Human Caprin family comprises two members, Caprin-1 and Caprin-2. Previously, we reported Caprin-2 as a new regulator of canonical Wnt signaling through a mechanism of facilitating LRP5/6 phosphorylation. HR1 domain is so far only observed in Caprin-1 and Caprin-2, and this domain shares no sequence similarities with any other known motifs, indicating that HR1 may perform a unique function.

We then tried the corresponding region of hCap2_HR1 (aa S102–K351) based on sequence alignment between hCaprin-2 and zCaprin-2, and this hCap2_HR1 protein was crystallized with significantly improved diffractions. Two molecules of hCap2_HR1 form an asymmetric dimer, with the overall structure roughly resembling the shape of a pair of "scissors" measuring ∼100 Å in height and ∼60 Å in width. The structure of hCap2_HR1 could be divided into two subdomains: a "blade"-like N-lobe (aa A112-L205) and a "bow"-like C-lobe (aa K206-P320). The parts of helices α3-2 and α3′ in the C-lobe of chains A and B, respectively, packed together forming a parallel coiled-coil dimer with the rest helices in the N-lobe forming two antiparallel dimers. The dimeric interface has a total buried area of 2414.4 Å2. Considering the theoretical MW of Cap2_HR1 being 29.2 kDa, we tend to conclude that Cap2_HR exists as a dimer in solution. Close to the junction of the N-lobe and the C-lobe, a cluster of basic residues aligned along the solve-exposed side of the coiled coil of the N-lobe. Surprisingly, we found that Cap2_HR1 binds specifically to phosphatidylinositol 4-phosphate (PI4P), and mutations targeting R200 and R201 in this basic cluster not only disrupt Caprin-2's association with PI4P but also lead to altered cellular localization as well as decreased activities of Caprin-2 in canonical Wnt signaling. WT hCap2_HR1 exhibited a binding affinity with PI4P (KD = 2.0 μm), which is about 70-fold higher than that of the double mutant R200E/R201E (KD = 152 μm).

> MDSPLQSTLSSAASPSQAYETYIENGLICLKHKIRNIEKKKLKLEDYKDRLKSGEHLNPDQLEAVEKYEEVLHNLEFAKELQKTFSGLSLDLLKAQKKAQRREHMLKLEAEKKKLRTMLQVQYVLQNLTQEHVQKDFKGGLNGAVYLPSKEMDYLIKFSKLTCPERNESLSVEDQMEQSSLYFWDLLEGSEKAVVGTTYKHMKDLLSKLLNSGYFESIPVPKNAKEKEVPLEEEMLIQSEKKTQLSKTESVKLEHHHHHH>MSDSSPTINFINFNQTGTCISLGTSKGFKIFNCEPFGKFYSEDSGGYAIVEMLFSTSLLALVGIGDQPALSPRRLRIINTKKHSIICEVTFPTSILSVKMNKSRLVVLLQEQIYIYDINTMRLLHTIETNPNPRGLMAMSPSVANSYLVYPSPPKVINSEIKAHATTNNITLSVGGNTETSFKRDQQDAGHSDISDLDQYSSFTKRDDADPTSSNGGNSSIIKNGDVIVFNLETLQPTMVIEAHKGEIAAMAISFDGTLMATASDKGTIIRVFDIETGDKIYQFRRGTYATRIYSISFSEDSQYLAVTGSSKTVHIFKLGHSMSNNKLDSDDSNME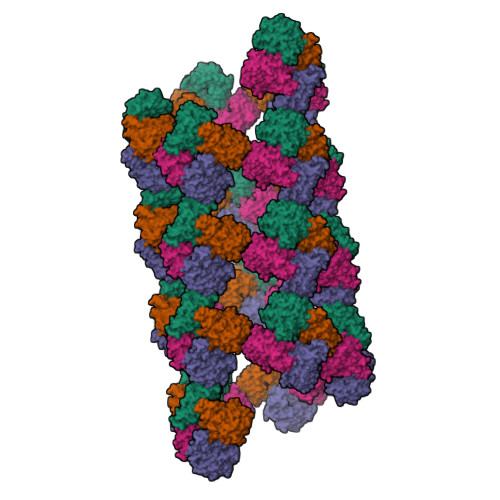EAAADDSSLDTTSIDALSDEENPTRLAREPYVDASRKTMGRMIRYSSQKLSRRAARTLGQIFPIKVTSLLESSRHFASLKLPVETNSHVMTISSIGSPIDIDTSEYPELFETGNSASTESYHEPVMKMVPIRVVSSDGYLYNFVMDPERGGDCLILSQYSILMD[4x]>[4x]HHHHHHMSMRDAVICEPVRTPIGRYGGMFRSLTAVDLGVTALKGLLERTGIAADQVEDVILGHCYPNSEAPAIGRVVALDAGLPITVPGMQVDRRCGSGLQAVIQACLQVRSGDHDLVVAGGAESMSNVAFYSTDMRWGGARTGVQIHDGLARGRTTAGGKFHPVPGGMLETAENLRREYHISRTEQDELAVRSHQRAVAAQSEGVLAEEIIPVPVRTRDGE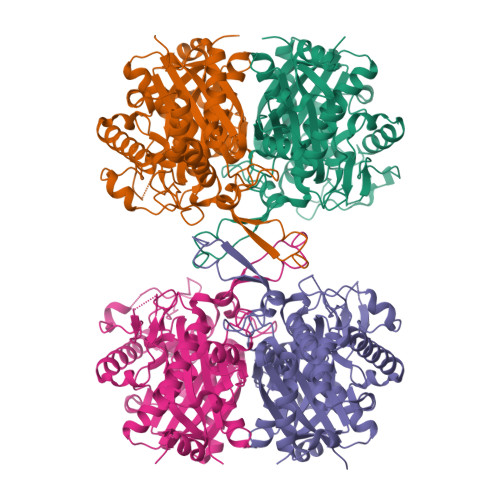ETISVDEHPRADTTVEALAKLKPVLLKQDPEATVTAGNSSGQNDAASMCIVTTPEKAAELGLKPLVRLVSWGSAGVAPDLMGIGPVPATEVALAKAGLTLADIDLIELNEAFAAQALAVMREWKFGEADHERTNVRGSGISLGHPVGATGGRMLATLARELHRREARYGLETMCIGGGQGLAAVFERVQEG>[2x]GPHMTRLGLEFFDQPAVPLARAFL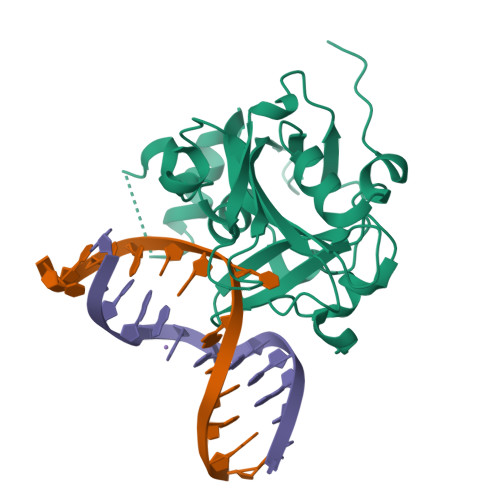GQVLVRRLPNGTELRGRIVETEAYLGPEDEAAHSRGGRQTPRNRGMFMKPGTLYVYIIYGMYFCMNISSQGDGACVLLRALEPLEGLETMRQLRSTLRKGTASRVLKDRELCSGPSKLCQALAINKSFDQRDLAQDEAVWLERGPLEPSEPAVVAAARVGVGHAGEWARKPLRFYVRGSPWVSVVDRVAEQDTQA> YCTLSSGFTTVDISMAVGRVVVRPSDPVGKILRKATFPINPNGSTLRCTSYSDTITAALTQNYPLSPLGNSIYSTNIPGIGIRLYREAENATNFSGYYPYTRSLTPGTTYNLAQGYFVVEIVKTADQTGSGTLVPGLYSRYYVNGHMDRPFLTSTVYGNAITIASSSHHHHHH

We identified two virulence pili independently critical to A. baumannii catheter-associated urinary tract infections, the chaperone-usher pathway pili Abp1 and Abp2. Further, their respective tip-adhesive proteins, the adhesins Abp1D and Abp2D, make use of large, distally oriented binding pockets to adhere to glycoproteins like fibrinogen, a wound-healing protein important in CAUTI pathogenesis. We demonstrate that Abp1D and Abp2D RBDs are structurally similar, and each binds fibrinogen and other relevant host glycoproteins important in CAUTI and other infections. These proteins share a common binding mechanism, using a large, distally oriented, and flexible pocket that recognizes a complex glycan receptor.

In Abp2DRBD, two 310 helices are present, one at the C-terminus and one between β strands 8 and 9. The C-terminal helix results from the six histidine tag added to this construct for purification. However, the 310 helix between β strands 8 and 9 forms the anterior loop of a large, open depression (>200 Å3) located at the distal end of the RBD relative to the linker to the pilin domain (and by extension, pilus rod). The carboxylic acid residues of the citrate are coordinated by the side chains of the amino acids R86, Y100, R102, and Y141. Y100 and R102 sit on the left-hand ridge of the binding site, while the base is composed of the Y141 side chain, which emanates from a β sheet on the opposite side of the receptor-binding domain core (β strand 13) and R86, situated on β strand 8. The R102 and Y141A mutations reduced binding relative to Abp2DRBD WT by approximately ~70% and ~90%, respectively. The crystal structure of Abp2DRBD shows that K34 forms a salt bridge with E87. Therefore, the K34A salt bridge seen in the Abp2D structure is holding the anterior loop down, keeping the pocket open. Subsequent analysis showed that equilibrium populations of Abp2DRBD skewed toward a larger pocket opening distance, indicating that the anterior binding pocket loop in Abp2DRBD is flexible but predominantly favors a more open conformation.>ASIPSSASVQLDSYNYDGSTFSGKIYVKNIAYSKKVTVVYADGSDNWNNNGNIIAASFSGPISGSNYEYWTFSASVKGIKEFYIKYEVSGKTYYDNNN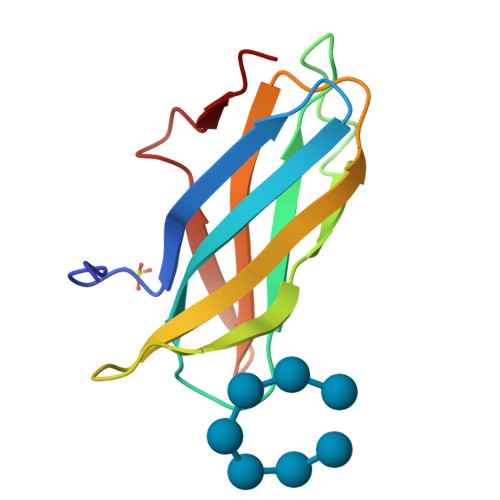SANYQVST[4x]>[2x]MSLQASGNTDQAALESAQARLAALSILVGAVGATGPGVMITIDDPGPGVAPEVMIDVINELRAAGAEAIQINDAHRSVRVGVDTWVVGVPGSLTVDTKVLSPPYSILAIGDPP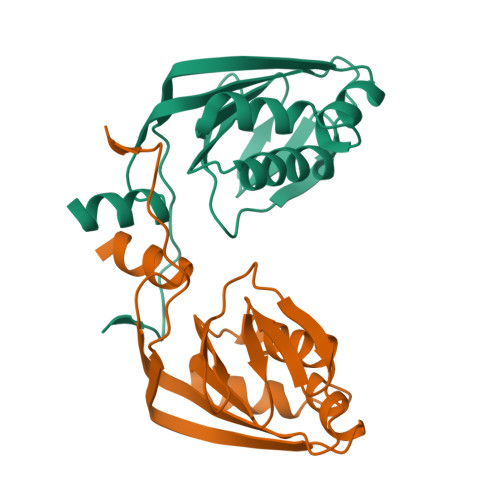TLAAAMNIPGGAQDGVKRVGGRMVVQQADRVDVTALRQPKQHQYAQPVKEGHHHHHH> MSQSNRELVVDFLSYKLSQKGYSWSQPMAAVKQALREAGDEFELRYRRAFSDLTSQLHITPGTAYQSFEQVVNELFRDGVNWGRIVAFFSFGGALCVESVDKEMQVLVSRIASWMATYLNDHLEPWIQENGGWDTFVDLYG;> APIRYEWDEFC

The anti-apoptotic (pro-survival) proteins of the BCL-2 family include BCL-2, BCL-XL, MCL-1, BCL-w and BFL-1/A1. These proteins bind to and sequester the apoptosis effectors, as well as the apoptosis sensitizers, BIM, BID, PUMA, NOXA, BAD, BMF, HRK and BIK5,6. An elongated hydrophobic groove is thus formed along the surface of BCL-2 and BCL-XL proteins, spanning approximately 20 Å to serve as the binding site for the amphipathic α-helical BH3 domains of their pro-apoptotic partners. Herein we present cyclic peptides (CPs) with nanomolar-level binding affinities to BCL-2 or BCL-XL, and further reveal the structural and functional mechanisms of how these CPs target two proteins in a fashion that is remarkably different from traditional small-molecule inhibitors.

From the BCL-2 targeted screening we obtained a CP annotated as cp2, which exhibited enhanced binding affinities to both BCL-2 (0.20 ± 0.01 μM) and BCL-XL (0.73 ± 0.18 μM) as measured by SPR. However, it appears cp2 is only 3.6-fold preferential for BCL-2 over BCL-XL, much lower than cp1’s > 19-fold selectivity to BCL-2. The electron density maps of cp2 and cp3 were all clearly defined. The overall three-dimensional structures of BCL-XL in complex with cp1, cp2 and cp3 are very similar (RMSD for all their Cα atoms between BCL-XL-cp1 and BCL-XL-cp2, BCL-XL-cp1 and BCL-XL-cp3, BCL-XL-cp2 and BCL-XL-cp3 are 0.216 Å, 0.199 Å and 0.171 Å, respectively). We again analyzed the key residues within 5 Å around these CPs, and found that there are more BCL-XL residues interacting with cp2 than cp1, in line with cp2’s larger interaction area (the buried interfaces of cp1 and cp2 to BCL-XL are 592.6 Å2 and 638.8 Å2). This finding correlates with the higher binding affinity of cp2 to BCL-XL (0.73 ± 0.18 μM) than that of cp1. Meanwhile it is noteworthy that the side chain of cp2-E6 can also interact with BCL-2 R110 and BCL-XL R103 residues, respectively. Therefore, this special interacting mode of cp2-E6 may partially explain the enhanced binding affinities of cp2 to both BCL-2 and BCL-XL, as well as its reduced selectivity to BCL-2 when compared with cp1.>MGGGPNTGRDKDHLLKYNVGDLVWSKVSGYPWWPCMVSADPLLHSYTKLKGQKKSARQYHVQFFGDAPERAWIFEKSLVAFEGEGQFEKLCQESAKQAPTKAEKIKLLKPISGKLRAQWEMGIVQAEEAASMSVEERKAKFTFLYVGDQLHLNPQVAK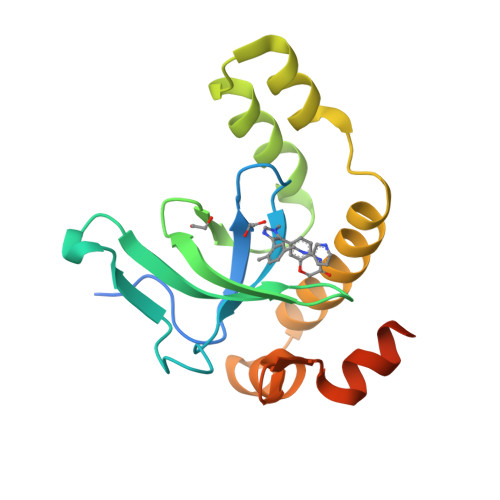EAGIAAEGGGENLYFQ[2x]>[2x]KMNESDIWFEEKLQEVECEEQRLRKLHAVVETLVNHRKELALNTAQFAKSLAMLGSSEDNTALSRALSQLAEVEEKIEQLHQEQANNDFFLLAE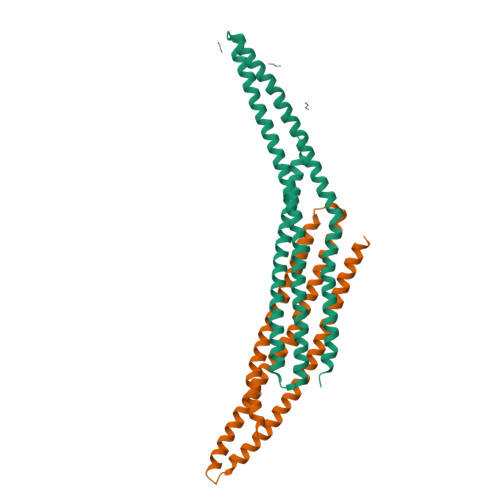LLSDYIRLLAIVRAAFDQRMKTWQRWQDAQATLQKKREAEARLLWANKPDKLQQAKDEILEWESRVTQYERDFERISTVVRKEVIRFEKEKSKDFKNHVIKYLETLLYSQQQLAKYWEAFLPEAKAIS;>DEVLFTGVKEVDDFFEQEKNFLINYYNRIKDSCVKADKMTRSHKNVADDYIHTAACLHSLALEEPTVIKKYLLKVAELFEKLRKVEGRVSSDEDLKLTELLRYYMLNIEAAKDLLYRRTKALIDYENSNKALDKARLKSKDVKLAEAHQQECCQKFEQLSESAKEELINFKRKRVAAFRKNLIEMSELEIKHARNNVSLLQSCIDLFKNN[2x]> MSFESKKPMRTWSH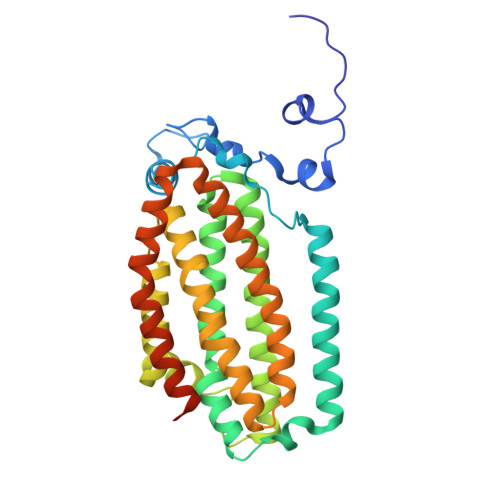LAEMRKKPSEYDIVSRKLHYSTNNPDSPWELSPDSPMNLWYKQYRNASPLKHDNWDAFTDPDQLVYRTYNLMQDGQESYVQSLFDQFNEREHDQMVREGWEHTMARCYSPLRYLFHCLQMSSAYVQQMAPASTISNCCILQTADSLRWLTHTAYRTHELSLTYPDAGLGEHERELWEKEPGWQGLRELMEKQLTAFDWGEAFVSLNLVVKPMIVESIFKPLQQQAWENNDTLLPLLIDSQLKDAERHSRWSKALVKHALENPDNHAVIEGWIEKWRPLADRAAEAYLSMLSSDILPAQYLERSTSLRASILTV> DCPSDWSSYEGHCYKPFSEPKNWADAENFC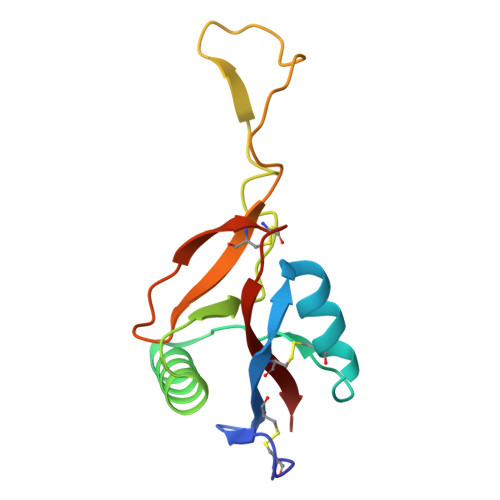TQQHAGGHLVSFQSSEEADFVVKLAFQTFGHSIFWMGLSNVWNQCNWQWSNAAMLRYKAWAEESYCVYFKSTNNKWRSRACRMMAQFVCEFQA>ARPCIPKSFGYSSVVCVCNATYCDSFDPPTFPALGTFSRYESTRSGRRMELSMGPIQANHTGTGLLLTLQPEQKFQKVKGFGGAMTDAAALNILALSPPAQNLLLKSYFSEEGIGYNIIRVPMASCDFSIRTYTYADTPDDFQLHNFSLPEEDTKLKIPLIHRALQLAQRPVSLLASPWTSPTWLKTNGAVNGKGSLKGQPGDIYHQTWARYFVKFLDAYAEHKLQFWAVTAENEPSAGLLSGYPFQCLGFTPEHQRDFIARDLGPTLANSTHHNVRLLMLDDQRLLLPHWAKVVLTDPEAAKYVHGIAVHWYLDFLAPAKATLGETHRLFPNTMLFASEACVGSKFWEQSVRLGSWDRGMQYSHSIITNLLYHVVGWTD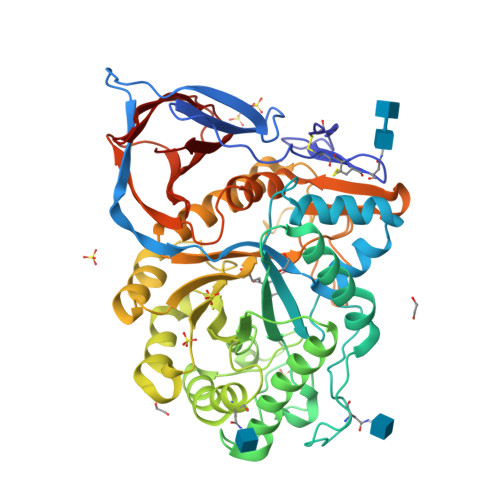WNLALNPEGGPNWVRNFVDSPIIVDITKDTFYKQPMFYHLGHFSKFIPEGSQRVGLVASQKNDLDAVALMHPDGSAVVVVLNRSSKDVPLTIKDPAVGFLETISPGYSIHTYLWHRQ[2x]> MAS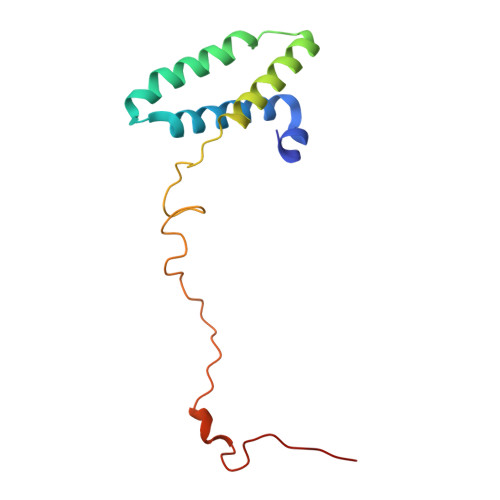EAVLRLPHKLRVMRMYRTGLKEIVNWSYGRHEFYPRANALRMEFEANKELSDREQIRKLVLHGEDLLARFRHWEPTIRSEFVGGTVYGVWPQHCKDVKFVPNPAYIDEFKQGDTVLLY> MKINNNFNIDSLIDNRDVAIVRGRKTDTFFKVFQVAPNIWVAPERYYGESLNINEDQKSDGGIYDSNFLLTNDEKDEFLQATVKILQRINNNVIGAKLLSLISTAIPFPYEYKPGDYRQTNYLVSKDNQHYYTANLVIFGPGTNIVENNAVYYKKEDSENGMGTMSEIWFQPFLTYKYDQFYVDPALELIKCLIKSLYYLYGIKPSDDLSIPYRLRSEFNSLEYSELDMVDFLISGGTDYKLLNTNPYWFTDNYFINAPKNFEKYKNDYETKIKNNNDIANSIKLYLEQKFKTNVQDIWELNLSYFSTEFEIMMPEIFNNALNHYHRKEYYVIDYFKNYNINGFINGQIKTILLLSKYNKNIINKPELIVNLINENNSVLMKSNIYGDGLKGTIGNFYAVYKIPYNIGDEYHINSSDSCLDNVDIKEIDNIPPINDADIYPYRKNCDPFTPVYNITETKEINTTIPFPVNYLQAQVTNSNDINLSSDFLKVISSKDRSLVYSFLDNTIDYLDSIKYDGPIDTDKKYYLWLKEIFRNYSFDMTETQEVNTLCGFNKVVPWLGKALNILNTGNSFIEEFKTLGPISLINKKENITMPKIEIDEIPNSMLNLSFKDLSENLFNIFSKNNSYFEKIYYDFLDQWWTQYYSQYFDLICMAKRSVLAQESLIKKIIQKKLSYLIGNSNISSDNLALMNLTTTNTLRDISNESQIAMNNVNNFLNNVAICVFQTNIYPKFISFMEQCINNINKNTREFIQKCTNITENEKLQLINQNIFSSLDFDFLNIENLKSLFNSETGLLIKEETSPYELVLYAFQEPGNNAIGDASGKNTSIEYSKDIGLVYGINSDALYLNGSNQSISFSNDFFENGLTNSFSIYFWLRNLGKDTIKSKLIGSKEDNCGWEIYFQDTGLVFNMIDSNGNEKNIYLSDVSNNSWHYIT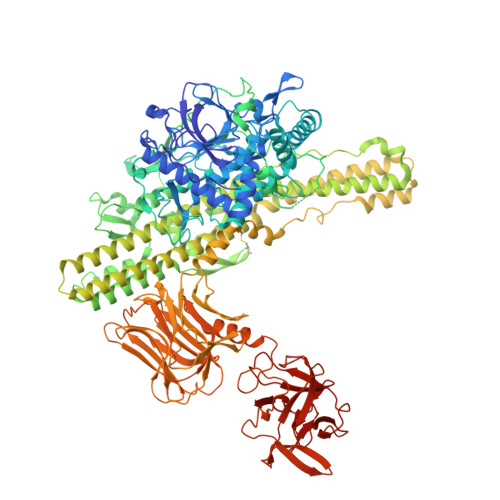ISVDRLKEQLLIFIDDNLVANESIKEILNIYSSNIISLLSENNPSYIEGLTILNKPTTSQEVLSNYFKVLNNSYIRDSSEERLEYNKTYQLYNYVFSENPIYEIKQNNNIYLTINNTNNLNLQVSKFKLLSINPNKQYVQKLDEVIISVLDNMEKYIDISEDNRLQLIDNKNNAKKMIISNDIFISNCLTLSYNGKYICLSMKDENHNWMICNNDMSKYLYLWSFK> MTLEKFVDALPIPDTLKPVQQSKEKTYYEVTMEECTHQLHRDLPPTRLWGYNGLFPGPTIEVKRNENVYVKWMNNLPSTHFLPIDHTIHHSDSQHEEPEVKTVVHLHGGVTPDDSAGYPEAWFSKDFEQTGPYFKREVYHYPNQQRGAILWYHDHAMALTRLNVYAGLVGAYIIHDPKEKRLKLPSDEYDVPLLITDRTINEDGSLFYPSAPENPSPSLPNPSIVPAFCGETILVNGKVWPYLEVEPRKYRFRVINASNTRTYNLSLDNGGDFIQIGSDGGLLPRSVKLNSFSLAPAERYDIIIDFTAYEGESIILANSAGCGGDVNPETDANIMQFRVTKPLAQKDESRKPKYLASYPSVQHERIQNIRTLKLAGTQDEYGRPVLLLNNKRWHDPVTETPKVGTTEIWSIINPTRGTHPIHLHLVSFRVLDRRPFDIARYQESGELSYTGPAVPPPPSEKGWKDTIQAHAGEVLRIAATFGPYSGRYVWHCHILEHEDYDMMRPMDIT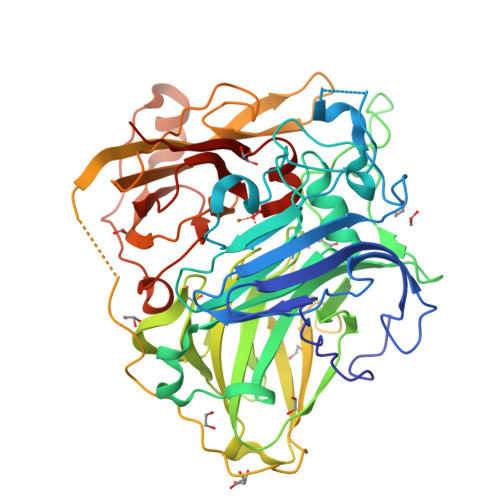DPHK>[2x]TSLKPTAIESCMVKFELSSSKWHMTSPKPHCVNTTSDGKLKILQSGTYLIYGQVIPVDKKYIKDNAPFVVQIYKKNDVLQTLMNDFQILPIGGVYELHAGDNIYLKFNSKDHIQKTNTYWGIILMPDLPFIS;>QPSVVEEPGCGPGKVQNGSGNNTRCCSLYAPGKEDCPKERCICVTPEYHCGDPQCKICKHYPCQPGQRVESQGDIVFGFRCVACAMGTFSAGRDGHCRLWTNCSQFGFLTMFPGNKTHNAVCIPEPLPTEQYGH[2x]

Glucocorticoid-induced tumor necrosis factor receptor-related protein (GITR) and GITR ligand (GITRL) are members of the tumor necrosis superfamily that play a role in immune cell signaling, activation, and survival. Upon binding to its ligand, GITRL, GITR produces costimulatory signals regulating T-cell proliferation and effector functions. Here we present structures of human and mouse GITR receptors bound to their cognate ligands. Both species share a receptor–ligand interface and receptor–receptor interface; the unique C-terminal receptor–receptor enables higher order structures on the membrane.

Although human GITRL shares more than 50% sequence similarity with mouse GITRL, mouse GITRL is a homodimer, suggesting a different 2:2 ligand/receptor stoichiometry. Similarly, we identified a mouse GITR variant C55S that can be produced recombinantly, referred to as mGITR for these structural and biophysical studies. We expressed mouse GITRL and determined the 3.2 Å structure of the dimeric mGITR–mGITRL complex to compare with the human complex. There is a cavity of negative potential from hGITRL D149 and E155 that positively charged K105 is positioned near. mGITR does not have a buried phenylalanine, but rather an isoleucine, and the glycines are conserved. mGITRL has basic charges (K147 and K153), while mGITR has a negative charge (D93), but this electrostatic interaction does not appear as favorable as hGITR. In CRD3, surprisingly, we find mouse and human receptors share a conserved membrane-proximal receptor–receptor interface, forming receptor homodimers between separate ligand–receptor complexes. In the C-terminus of the ligand, we see the previously reported strand swapping in mouse GITRL, but not in human GITRL, when ligands are complexed with their cognate receptors. In contrast, the loop rearrangements that occur upon GITR binding GITRL do not result in any allosteric affects at the dimer interface and the apo mGITRL dimer and receptor-bound mGITRL dimer are effectively superimposable. When considering the stoichiometry of the receptor–ligand complex in the context of the observed receptor–receptor interactions, the overall effect is in the crystallographic assembly mouse receptor–ligand complexes form a linear chained structure, while human receptor–ligand complexes form a tetrameric assembly. As a result, preclinical murine in vivo studies with agonist antibodies that engage mGITR as a dimer might exhibit different behavior than agonist antibodies that engage trimeric human GITR.> MAPGCKTELRSVTNGQSNQPSNEGDAIKVFVRIRPPAERSGSADGEQNLCLSVLSSTSLRLHSNPEPKTFTFDHVADVDTTQESVFATVAKSIVESCMSGYNGTIFAYGQTGSGKTFTMMGPSESDNFSHNLRGVIPRSFEYLFSLIDREKEKAGAGKSFLCKCSFIEIYNEQIYDLLDSASAGLYLREHIKKGVFVVGAVEQVVTSAAEAYQVLSGGWRNRRVASTSMNRESSRSHAVFTITIESMEKSNEIVNIRTSLLNLVDLAGSERQKDTHAEGMRLKEAGNINRSLSCLGQVITALVDVGNGKQRHVCYRDSKLTFLLRDSLGGNAKTAIIANVHPGSRCFGETLSTLNFAQRAKLIKNKAVVNEDTQG;> MANVPWAEVCEKFQAALALSRVELHKNPEKEPYKSKYSARALLEEVKALLGPAPEDEDERPEAEDGPGAGDHALGLPAEVVEPEGPVAQRAVRLAVIEFHLGVNHIDTEELSAGEEHLVKCLRLLRRYRLSHDCISLCIQAQNNLGILWSEREEIETAQAYLESSEALYNQYMKEVGSPPLDPTERFLPEEEKLTEQERSKRFEKVYTHNLYYLAQVYQHLEMFEKAAHYCHSTLKRQLEHNAYHPIEWAINAATLSQFYINKLCFMEARHCLSAANVIFGQTGKISATEDTPEAEGEVPELYHQRKGEIARCWIKYCLTLMQNAQLSMQDNIGELDLDKQSELRALRKKELDEEESIRKKAVQFGTGELCDAISAVEEKVSYLRPLDFEEARELFLLGQHYVFEAKEFFQIDGYVTDHIEVVQDHSALFKVLAFFETDMERR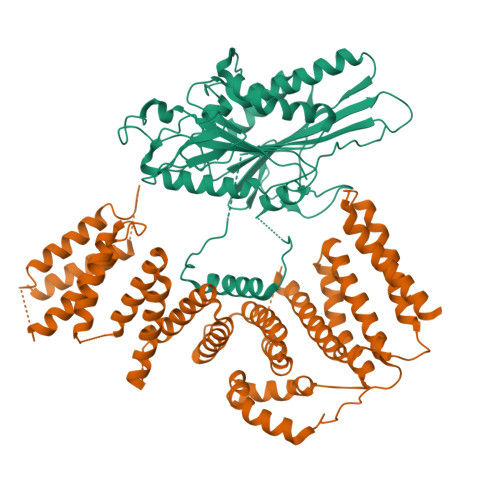CKMHKRRIAMLEPLTVDLNPQYYLLVNRQIQFEIAHAYYDMMDLKVAIADRLRDPDSHIVKKINNLNKSALKYYQLFLDSLRDPNKVFPEHIGEDVLRPAMLAKFRVARLYGKIITADPKKELENLATSLEHYKFIVDYCEKHPEAAQEIEVELELSKEMVSLLPTKMERFRTKMALT>MAAKQGSFRHGILEKRERLLSNNGFSDFRFTDIESNDLLENENCGRRTRLCCCCSCGNLSEKISGVYDDAKDVARKAWEMGVSDPRKIVFSAKIGLALTIVALLIFYQEPNPDLSRYSVWAILTVVVVFEFTIGATLSKGFNRALGTLSAGGLALGMAELSTLFGDWEEIFCTLSIFCIGFLATFMKLYPSMKAYEYGFRVFLLTYCYILISGFRTGQFIEVAISRFLLIALGAGVSLGVNMFIYPIWAGEDLHNLVVKNFMNVATSLEGCVNGYLRCLEYERIPSKILTYQASEDPVYKGYRSAVESTSQEESLMSFAIWEPPHGPYKSFNYPWKNYVKLSGALKHCAFTVMALHGCILSEIQAPEERRQVFRQELQRVGVEGAKLLRELGEKVKKMEKLGPVDLLFEVHLAAEELQHKIDKKSYLLVNSECWEIGNRATKESEPQELLSLEDSDPPENHAPPIYAFKSLSEAVLEIPPSWGEKNHREALNHRPTFSKQVSWPARLVLPPHLETTNGASPLVETTKTYESASALSLATFASLLIEFVARLQNVVDAFKELSQKANFKEPEIVTTGTDVEFSGERVGLGQKIRRCFGM[2x]

In plant cells, ALMTs are key plasma and vacuolar membrane-localized anion channels regulating plant responses to the environment. Among the different ion transporters and ion channels localized in the vacuolar membrane, the ion channels of the aluminum-activated malate transporter (ALMT) family play a key role for the transport of chloride and malate during stomata opening/closure. ALMTs are also involved in transporting various anion including chloride, nitrate, fumarate, tartrate, citrate, and malate. Here we report the cryo-EM structures of ALMT9 from Arabidopsis thaliana (AtALMT9), a malate-activated vacuolar anion channel, in plugged and unplugged lipid-bound states.

From the CHS-supplemented dataset 1 with no malate and dataset 2 with 10 mM malate, we unequivocally identified CHS densities in the lateral fenestrations and phospholipid (PL) densities in the pore (hereinafter called as “pore lipid”) in two classes. The only difference observed between the datasets 1 and 2 was the presence of a malate density in the pore of the dataset 2. In the CHS-supplemented datasets 1 and 2, we identified two distinct classes in the sterol mimic-bound state: “sterol 1” when one pore lipid tail of the sterol mimic (CHS) is in the fenestrations and “sterol 2” when two pore lipid tails of the sterol mimic (CHS) are in the fenestrations. Unexpectedly, we observed that the succinate head group of CHS interacted with several residues. Since the succinate group was the key structural moiety to differentiate CHS from native cholesterols, these interactions were likely to present artificial features and to inhibit pore lipid expulsion (described later). Similarly, the succinate head group of CHS in the lower fenestrations occupied the S3 region interacting with W120, Y208, and R226. These observations indicate that phosphate groups of PL and the dicarboxylic moieties (malate and succinate head group of CHS) compete with each other for malate binding sites S0, S1, and S3. The sterol mimic-bound and pore lipid-bound classes represent plugged states in which the pore is blocked by the head groups of one or two pore lipids. Additionally, the TMD of the sterol mimic-bound classes is similar with those of the pore lipid-bound and peripheral lipid-bound classes, suggesting that plant sterols may contribute to the regulation of the clade 2 ALMTs.>[4x]MNEYAPLRLHVPEPTGRPGCQTDFSYLRLNDAGQARKPPVDVDAADTADLSYSLVRVLDEQGDAQGPWAEDIDPQILRQGMRAMLKTRIFDSRMVVAQRQKKMSFYMQSLGEEAIGSGQALALNRTDMCFPTYRQQSILMARDVSLVEMICQLLSNERDPLKGRQLPIMY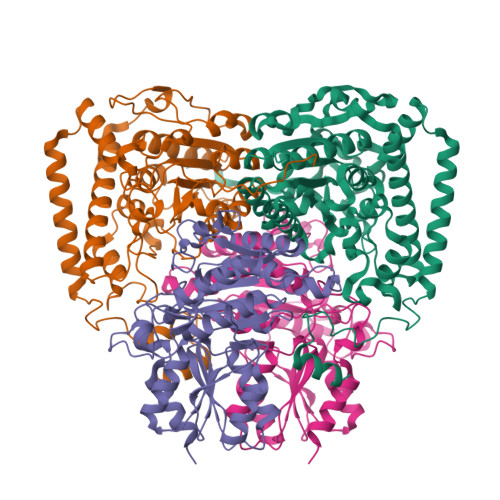SVREAGFFTISGNLATQFVQAVGWAMASAIKGDTKIASAWIGDGATAESDFHTALTFAHVYRAPVILNVVNNQWAISTFQAIAGGESTTFAGRGVGCGIASLRVDGNDFVAVYAASRWAAERARRGLGPSLIEWVTYRAGPHSTSDDPSKYRPADDWSHFPLGDPIARLKQHLIKIGHWSEEEHQATTAEFEAAVIAAQKEAEQYGTLANGHIPSAASMFEDVYKEMPDHLRRQRQELGV;>MATTTMTMIQALRSAMDVMLERDDNVVVYGQDVGYFGGVFRCTEGLQTKYGKSRVFDAPISESGIVGTAVGMGAYGLRPVVEIQFADYFYPASDQIVSEMARLRYRSAGEFIAPLTLRMPCGGGIYGGQTHSQSPEAMFTQVCGLRTVMPSNPYDAKGLLIASIECDDPVIFLEPKRLYNGPFDGHHDRPVTPWSKHPHSAVPDGYYTVPLDKAAITRPGNDVSVLTYGTTVYVAQVAAEESGVDAEVIDLRSLWPLDLDTIVESVKKTGRCVVVHEATRTCGFGAELVSLVQEHCFHHLEAPIERVTGWDTPYPHAQEWAYFPGPSRVGAALKKVMEV[4x]> GDVEEAIERAVVHVADTMRSGPSNSASVPALTAVETGHTSQVTPSDTMQTRHVKNYHSRSESTVENFLGRSACVYMEEYKTTDNDVNKKFVAWPINTKQMVQMRRKLEMFTYLRFDMEVTFVITSRQDPGTTLAQDMPVLTHQIMYVPPGGPIPAKV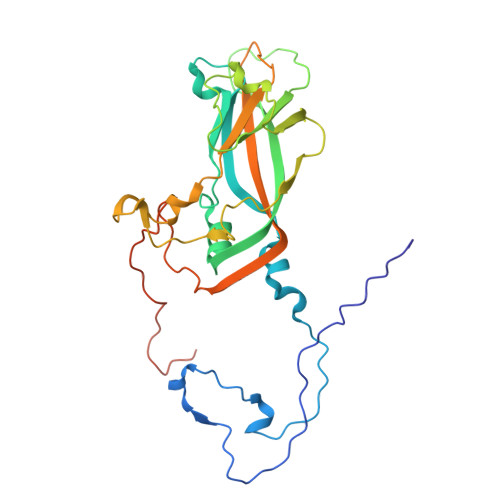DDYAWQTSTNPSIFWTEGNAPARMSIPFISIGNAYSNFYDGWSNFDQRGSYGYNTLNNLGHIYVRHVSGSSPHPITSTIRVYFKPKHTRAWVPRPPRLCQYKKAFSVDFTPTPITDTRKDINTVTTVAQSRRRGDMSTLNTH> MARARGRGRRDLKSEINIVPLLDVLLVLLLIFMATAPIITQSVEVDLPDATESQAVSSNDNPPVIVEVSGIGQYTVVVEKDR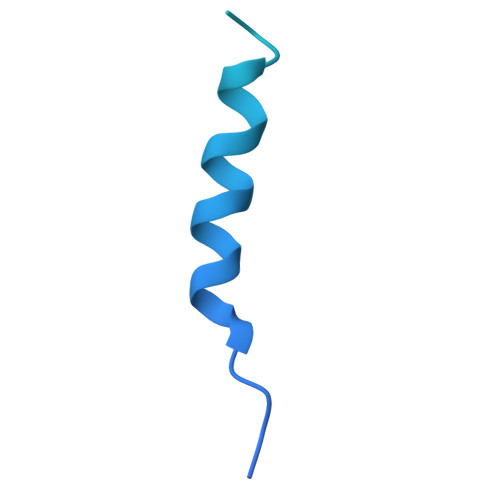LERLPPEQVVAEVSSRFKANPKTVFLIGGAKDVPYDEIIKALNLLHSAGVKSVGLMTQPILEHHHHHHHH>[2x]VAQISPQYPMFTVPLPIPPVKQPRLTVTNPVNGQEIWYYEVEIKPFTHQVYPDLGSADLVGYDGMSPGPTFQVPRGVETVVRFINN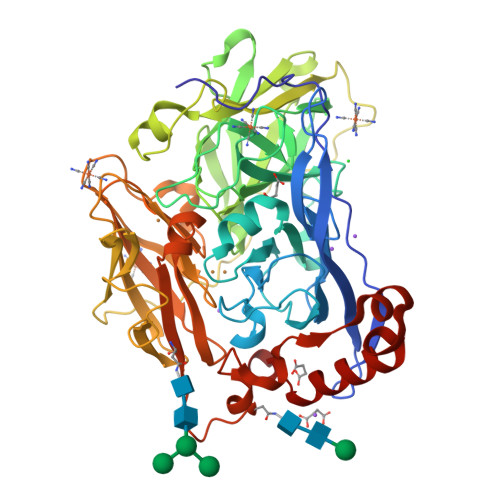AEAPNSVHLHGSFSRAAFDGWAEDITEPGSFKDYYYPNRQSARTLWYHDHAMHITAENAYRGQAGLYMLTDPAEDALNLPSGYGEFDIPMILTSKQYTANGNLVTTNGELNSFWGDVIHVNGQPWPFKNVEPRKYRFRFLDAAVSRSFGLYFADTDAIDTRLPFKVIASDSGLLEHPADTSLLYISMAERYEVVFDFSDYAGKTIELRNLGGSIGGIGTDTDYDNTDKVMRFVVADDTTQPDTSVVPANLRDVPFPSPTTNTPRQFRFGRTGPTWTINGVAFADVQNRLLANVPVGTVERWELINAGNGWTHPIHIHLVDFKVISRTSGNNARTVMPYESGLKDVVWLGRRETVVVEAHYAPFPGVYMFHCHNLIHEDHDMMAAFNATVLPDYGYNATVFVDPMEELWQARPYELGEFQAQSGQFSVQAVTERIQTMAEYRPYAAADE> GAMGEQIFYWSPAKHWRMSDEGVVIGESTYTGMILEWFPEFYFFAQTGVTINRLLERFSSGSEKEANEILELLIQDRVLVEGILPPREVFSPQEGLFVNPYSEQIRYSKEALDYYVSEQLNRTHAACRSTKIQLETSGALPDIIQKRRSCRRFDMKTPVSFATFSNLLSSLKQRKEDKILYNYASAGGLYPIDVFVYVKPRRVEGVKAGFYYFNPADHSLVLVNNIDQVIKDDHELINQDIFAQSAFSVYLVYNARASMPKYGAAGYFYACIEAGIITATLNMVAEDLNVGLCSIGHMNFEEIQTFLKLEDHQVILHAIEGGLKIDGAAAENLYFQ

The bacillamide biosynthetic pathway is a common, three-protein system, with a decarboxylase that prepares an NRPS substrate, an NRPS, and an oxidase. The oxidase is shown to perform dehydrogenation of the thiazoline in the peptide intermediate while it is covalently attached to the NRPS, as the penultimate step in bacillamide D synthesis. The oxidase forms a stable complex with the NRPS and dimerizes it. We visualized co-complexes of the oxidase bound to the elongation module of the NRPS using X-ray crystallography and cryo-EM.

The structure of BmdC shows it to be a dimer of di-domain protomers. A single copy of BmdC is present in the asymmetric unit, and the adjacent symmetrically related copy completes the biological dimer. The small N-terminal domain contains 96 residues and features a winged helix–turn–helix motif (wHTH) with a very small β-sheet. A DALI41 structural similarity search reveals this domain to be similar to the precursor peptide recognition elements (RRE) in ribosomally synthesized post-translationally modified peptide (RiPP) processing enzymes with Z-scores ranging from 5.3 to 6.5 and rmsd values of 2.0–2.9 Å over 61–69 alpha carbons. BmdC contains a 45-residue loop segment between the RRE-like (RREL) and Ox domains, that wraps around the Ox domain of the other protomer. The loop contributes 1764.3 Å2 of the total 5777.3 Å2 per-protomer surface area buried by BmdC dimerization. The electron density maps showed very strong density for flavin mononucleotide (FMN). One protomer contributes to most of the side-chain interactions, with both the FMN phosphate, (through Arg145, Arg146 and Ser147) and the catalytic isoalloxazine rings (hydrogen bonding of Arg149 with FMN N1 and O2, Asn236 with N3 and O4, plus Gly294 with N5; analogous to interactions observed in flavin reductase P51). The conserved active-site Tyr260 points toward the FMN in each protomer. There is room for the thiazole ring to bind between this Tyr260 residue and the catalytic FMN N5 atom; a glycine from the crystallization buffer is observed occupying this site.1-{6-[(3R)-3-methylmorpholin-4-yl]-2-(methylsulfanyl)pyrimidin-4-yl}cyclopropane-1-sulfonimidoamide | C13 H21 N5 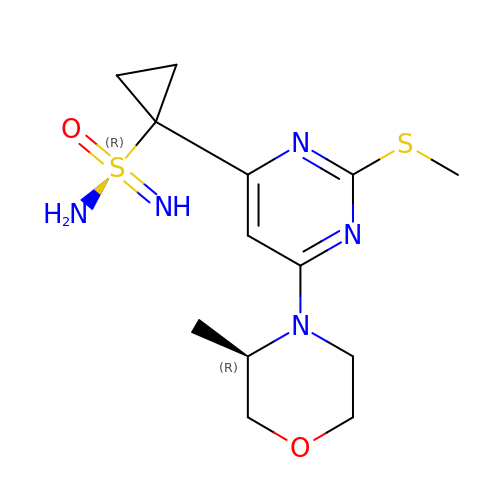O2 S2 | XGFQEZBAAOLAMH-SECBINFHSA-N>MGSSHHHHHHSSGLVPRGSHSDEVDAHMSVASAVEVGVGEDEEEGVEEEEEEVEAVVMPERYALGGACRVLAGMPAPLGATALDGGVNFAVYSAGASAASLCLFTPDDLEADEVTEEVPLDPLFNRTGNVWHVFIEGELHNMLYGYRFDGMFAPHCGQYFDVSNVVVDPYAKAVISRGEYGVPGPGGDCWPQMAGMIPLPYSTFDWQGDLPLRYPQKDLVIYEMHLRGFTKHSSSNVEHPGTYIGAISKLDYLKELGVNCVELMPCHEFNELEYFSCSSKMNFWGYSTINFFSPMIRYSSGGIRNCGRDAINEFKTFVREAHKRGIEVIMDVVFNHTAEGNEKGPILSFRGIDNSTYYMLAPKGEFYNYSGCGNTFNCNHPVVREFIVDCLRYWVTEMHVDGFRFDLASIMTRGCSLWDPVNVYGSPVEGDMTTTGTPLATPPLIDMISNDPILGDVKLIAEAWDAGGLYQVGQFPHWKIWSEWNGKYRDIVRQFIKGTDGFAGGFAECLCGSPHLYQAGGRKPWHSINFVCAHDGFTLADLVTYNKKYNSSNGEDNRDGENHNLSWNCGEEGEFAGLSVKRLRKRQMRNFFVSLMVSQGVPMFYMGDEYGHTKGGNNNTYCHDHYVNYFRWDKKEESSDLQRFCSLMTKFRKQCE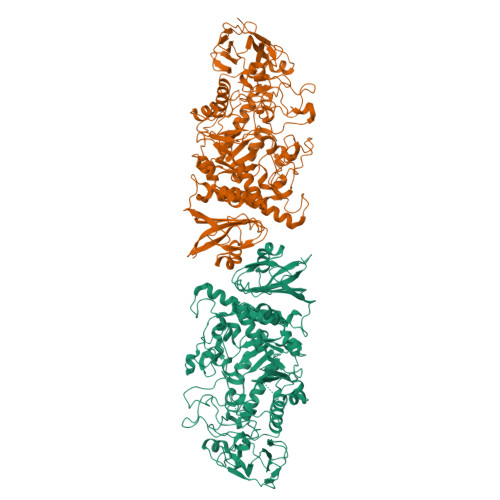SLGLADFPTAQRLHWHGHQPGKPDWSETSRFVAFSTKDETKGEIYVAFNASHLPAVVGLPERPGYRWEPLVDTGKPAPYDFLTDDLPDRAHAVHLFSHFLNSNLYPMLSYSSIILELQPDD[2x]>TADELVFFVNGKKVVEKNADPETTLLAYLRRKLGLRGTKLGCGEGGCGACTVMLSKYDRLQDKIIHFSANACLAPICTLHHVAVTTVEGIGSTKTRLHPVQERIAKSHGSQCGFCTPGIVMSMYTLLRNQPEPTVEEIEDAFQGNLCRCTGYRPILQGFRTFAK[2x];>PKQLRFEGERVTWIQASTLKELLDLKAQHPEAKLVVGNTEIGIEMKFKNQLFPMIICPAWIPELNAVEHGPEGISFGAACALSSVEKTLLEAVAKLPT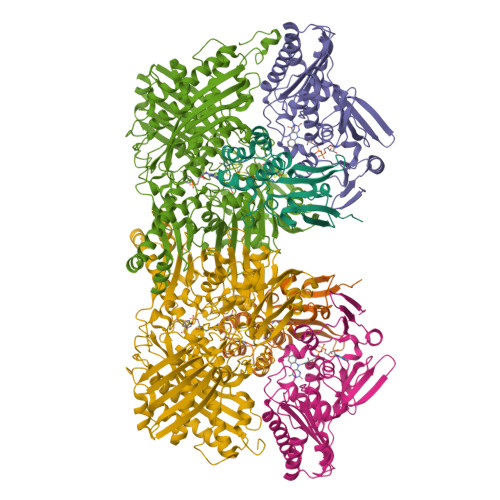QKTEVFRGVLEQLRWFAGKQVKSVASLGGNIITASPISDLNPVFMASGTKLTIVSRGTRRTVPMDHTFFPSYRKTLLGPEEILLSIEIPYSREDEFFSAFKQASRREDDIAKVTCGMRVLFQPGSMQVKELALCYGGMADRTISALKTTQKQLSKFWNEKLLQDVCAGLAEELSLSPDAPGGMIEFRRTLTLSFFFKFYLTVLKKLG[2x];>[2x]DTVGRPLPHLAAAMQASGEAVYCDDIPRYENELFLRLVTSTRAHAKIKSIDVSEAQKVPGFVCFLSADDIPGSNETGLFNDETVFAKDTVTCVGHIIGAVVADTPEHAERAAHVVKVTYEDLPAIITIEDAIKNNSFYGSELKIEKGDLKKGFSEADNVVSGELYIGGQDHFYLETHCTIAIPKGEEGEMELFVSTQNAMKTQSFVAKMLGVPVNRILVRVKRMGGGFGGKETRSTLVSVAVALAAYKTGHPVRCMLDRNEDMLITGGRHPFLARYKVGFMKTGTIVALEVDHYSNAGNSRDLSHSIMERALFHMDNCYKIPNIRGTGRLCKTNLSSNTAFRGFGGPQALFIAENWMSEVAVTCGLPAEEVRWKNMYKEGDLTHFNQRLEGFSVPRCWDECLKSSQYYARKSEVDKFNKENCWKKRGLCIIPTKFGISFTVPFLNQAGALIHVYTDGSVLVSHGGTEMGQGLHTKMVQVASKALKIPISKIYISETSTNTVPNSSPTAASVSTDIYGQAVYEACQTILKRLEPFKKKNPDGSWEDWVMAAYQDRVSLSTTGFYRTPNLGYSFETNSGNAFHYFTYGVACSEVEIDCLTGDHKNLRTDIVMDVGSSLNPAIDIGQVEGAFVQGLGLFTLEELHYSPEGSLHTRGPSTYKIPAFGSIPTEFRVSLLRDCPNKKAIYASKAVGEPPLFLGASVFFAIKDAIRAARAQHTNNNTKELFRLDSPATPEKIRNACVDKFTTLCVTGAPGNC>[3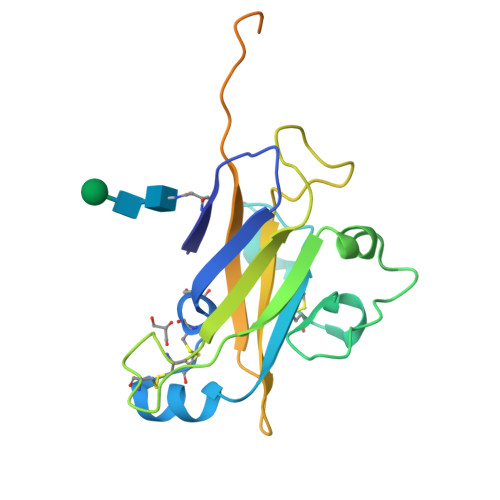x]ASHLIINVTRSDSPQTITFDACLVIPCGDLQSQRQLAAAEKYLCPSEADASTLFSFPFCHTWEYVVWTTQRQDWVPSQDFPLAVLKPYIHFTKGIAPPNCRYNQCNPVQISITIPTLQDSSPTLNRFYGMGADVRGKDPIGFFELHLSTSPSLISPRLSGAYPYDVPDYAGAGLEVLFQGPGGAHHHHHHHHGGAHHHHHH>MAKPQVTILATGGTIAGSGESSVKSSYSAGAVTVDKLLAAVPAINDLATIKGEQISSIGSQEMTGKVWLKLAKRVNELLAQKETEAVIITHGTDTMEETAFFLNLTVKSQKPVVLVGAMRPGSSMSAD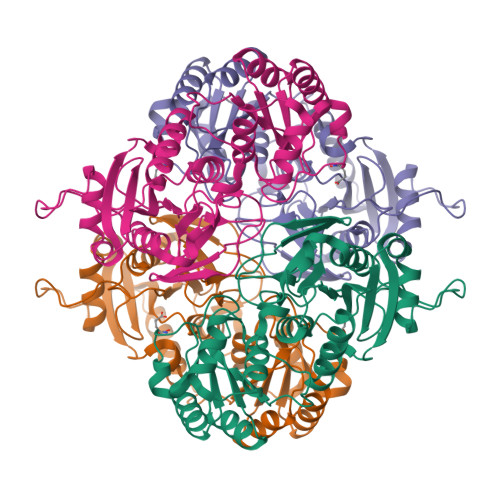GPMNLYNAVNVAINKASTNKGVVIVMNDEIHAAREATKLNTTAVNAFASPNTGKIGTVYYGKVEYFTQSVRPHTLASEFDISKIEELPRVDILYAHPDDTDVLVNAALQAGAKGIIHAGMGNGNPFPLTQNALEKAAKSGVVVARSSRVGSGSTTQEAEVDDKKLGFVATESLNPQKARVLLMLALTKTSDREAIQKIFSTY[4x]>CDLNINDDPNYPMNDQVTADLIFPSISASIASAVGGEIYNYAGFFAQYYEQKPESNQYNTLCEYTFTESSQQMDYSYRILFAGALEDAKQVLEKTTNPADRFATTILRAYAFQIMVDNTSDSPYSEALQGNANATPKWDTGETVYKGILGEIDAAEAALDGSGMDVPDLIFNKNIAQWKGFANALRLRMYLRFIDANIDAASYTEKVKTLVQNNEFFTGDVKLDCFLDETDKRNPWYNTNAVGLTGNHCAAYPLVSYLSSTGDPRIAYGISKTDADGKYVGQLPGGKTHMQSILGTDNWKNKNVSAIDYSIGATKPVYFFTQAELQFLIAEVYARFHNDDANAKSAYEAGVTADFAVRGFAGQENTILEGACAWSAASTQADKLNLIYMQKWVSLFYMDHMEAWSEIRRTDCPKLSSYSAAQIQASESVYTPGELVAPWTNGLEAGGLMKRMTYPLSARQQNVNTPAGVPGSTPVWWDIK[2x];>MQTQEVAIKPNLKVVLRSDAQQIDEVVVTAMGIKRSEKALGYAATSVGGEKIAESRTSDVMSSLAGKIAGVQISSTSSDPGASNSVIIRGVSSLSGTNQPLYVVDGVPLNNSTVYSTDGLNSGYDFGNGANAINPDDVANMTILKGAAATALYGSRAANGVVMITTKSGRKEKGVGIEYNGGVQWSTVLRLPEFQNEFGMGWNGNHTELENGSWGPRFDGSMQLWGNVYNNSQKLKPYVAMPDNIKDFFDAGFRYSNSLSFNGATDKSDYYVSFSQISDDGMIPTDADSYDKYTFSARGSHKAGALTFSSSLNYAYQKNNFATTGQGLSMLNSLYQTPRDISIIGLEDQNDPFNTPGYYYTPYGVMNPYYILNNYLNEYESERFYGKFQLDYEFLKYFKFTYRMGLDTTTGQSDKGKPNLYALYYEGTPNGEGQGSSSPFSGETGQYSEQITRRREINQDIMVNFNMPVNDFNINALVGFNGNERKVSYQYSEVNDLTIPTWFNLKNSGKTPIVEQHMELRRLMGVFGQFEGSWKNMLYLTVTARNDWSSTLPKENRSFFYPGITGSFIFSELLNDNLQDVITFGKIRASWGKTGNDADVYMVNPVYAQSSNRIPFGSLTFPLGGVNAYSAGNVLGSNTLSPEMTTESEVGLNMAFFKNRLSFDVSYYNRNTDKQIFSLAMDPASGYTAQNMNLGKIRNRGIELLISGTPIRTKDFSWELTWNFTKNWSKVISLPEELGGITTIYGLNGGTSMYAITGMPVGVFKAQVAERDPQGRIVVNSSTGLPVEASEFGICGDMNNKYQMGVSTNLKYKGISLGIDFDIRQGGVMYSRTKDINYFTGNAIQTAYNDRNPLIVPNSVNKIVNGENVTYVENTTPITSSNIYKYWGDGGSDMGSCFLVDKSYVKLRSVVLGWDLPKR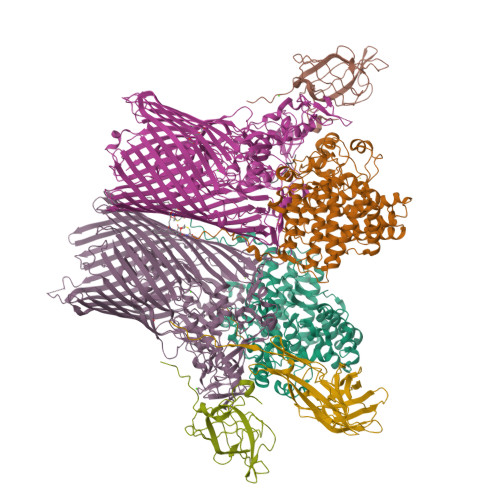WLAKTPFQAVKVSAYGNNLFVWTPSSNTFIDPEMTSFGNDLEGNYGEYTANPSSRRFGFNLMVKF[2x];>[2x]CDNDTEPGGTAVEKMAGDWWVTVNAFIDGKEVEDPFGAGHLQMSTYNTASNSETEMWLDDLGNFWEYKLKVNVNYAARTFSTTGFVDNVTYESKVKITDGKVLEKAATTPSGMPADSIVYMVQFDDDEDGLTYKVSGFRRTGFPADDF;> CDKSTDDTSKVTYFVTLEREGDEKIVLEKGQPFVEPGYYAEMNGEDITESVQIKGSVDVNTPGIYNLVYAAYNEDGFAKTFTRTVYVADNTASPLKSGIYTVAEGSKRTAPSVVAFSGYEIVIFQMEPGIFYISDFLGGWYDQRAGYGPDYAMVGKFELNDDNTITPLESYVAGWGDSMDQMTNTLLDPATGTLKWTVAYAGQLSFDIIVKQ;> GGGGGGGGGG;> GGGGGGGGG>MSEENKPVEREEDTVRYEIVNNVAWVYYNRPTKRNAQSPKLNRQMLKVLTELEFRDDVGVLVLGGEGPAWCAGMDLKEYFRETEAEGLAGTRKAQREAYTWWERL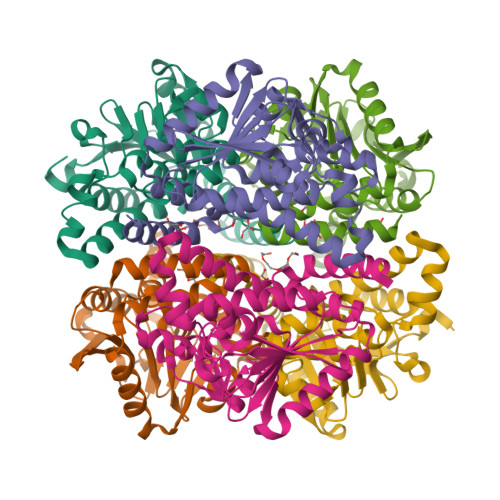RWYQKPTIAMVHGWCFGGAYGPLFACDLAFAADEAQFGLSEVNWGILPGGGATKVAVDLMPMRVAMYHAMMGENLSGQDAARYNLVNESMPADQLKARVKQVAETLIQKNWATVKYTKDAVRRVKEMTYDNAEDYLIRLQEGLNWFDKSDGRHVAMKQFLDDKTFKPGLGHYDKTKTEVLEHHHHHH[2x]>GSQQGKFDTKGIESTDEAKMSFLVTLNNVEVCSENISTLKKTLESDCTKLFSQGIGGEQAQAKFDSCLSDLAAVSNKFRDLLQEGLTELNSTAIKPQVQPWINSFFSVSHNIEEEEFNDYEANDPWVQQFILNLEQQMAEFKASLSPVIYDSLTGLMTSLVAVELEKVVLK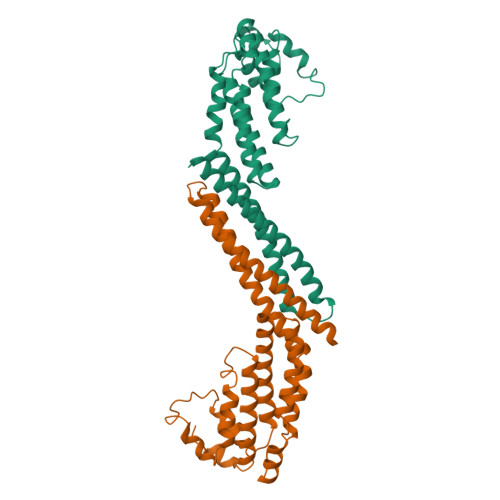STFNRLGGLQFDKELRSLIAYLTTVTTWTIRDKFARLSQMATILNLERVTEILDYWGPNSGPLTWRLTPAEVRQVLALRIDFRSEDIKRLRL[2x]>[2x]MHLICQSGDVLSARYEIVDTLGEGAFGKVVECIDHKAGGRHVAVKIVKNVDRYCEAARSEIQVLEHLNTTDPNSTFRCVQMLEWFEHHGHICIVFELLGLSTYDFIKENGFLPFRLDHIRKMAYQICKSVNFLHSNKLTHTDLKPENILFVQSDYTEAYNPKIKRDERTLINPDIKVVDFGSATYDDEHHSTL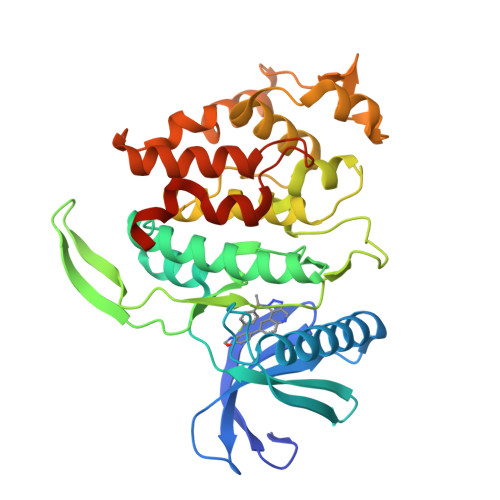VSTRHYRAPEVILALGWSQPCDVWSIGCILIEYYLGFTVFPTHDSKEHLAMMERILGPLPKHMIQKTRKRKYFHHDRLDWDEHSSAGRYVSRACKPLKEFMLSQDVEHERLFDLIQKMLEYDPAKRITLREALKHPFFDLLKKSILEHHHHHH>[2x]MKYNTGAGTVPEQLNVHLVPHSHDDVGWLKTVDQYYVGSENYIQEACVENVLDSVVMSLQRDPNRKFVFGEMAFFHRWWLEQTPETKELVRKLVKAGQLEFVNGGWCMHDEATTHYIDMIDHTTLGHRFIQEQFNKIPRAGWQIDPFGHSAVQGYLLGAELGFDSVHFARIDYQDREKRKAEKSLEVVWRGSKTFGSSAQIFANAFPGHYGP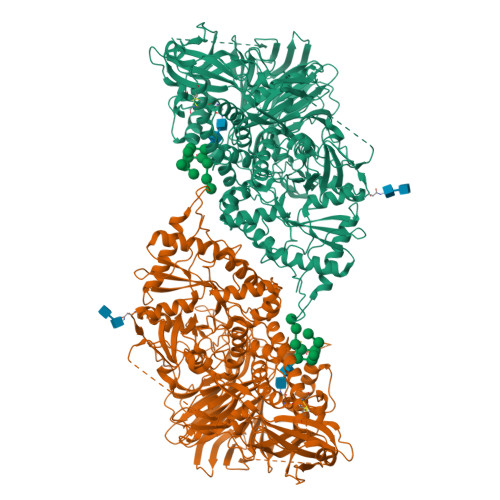PNGFNFEVRNNFVPLQDDPRLFDTNVEERVQNFIDAALTQAKITRTNHIMWTMGDDFQYQYAESWFKQMDKLIHHVNKDGRVNALYSTPSIYTEAKNAANQTWPLKIDDYFPYADGRNAYWTGFYTSRSALKDYVRMLSGYYLATRQLGFFAGKKSTKYHAFDLADALGIAQHHDAVSGTAKQHTTNDYAKRLAIGASKAEAVVSSSLACLTSKQSADQCSAPASAFSQCHLFNISYCPPTESSIPDDKSLVVVVYNPLGWSRNEIVRIPVNDANLVVKDSSGNKLEVQYVEMDDVTANLRSFYVKAYEGEVPKDADVYWSLFKASVPPLGWSTYFISEATGKGTRNALTLSQKGETLNIGPGDLKMSFSSLTGQLKRMYNSKTGVDIPIQQNYLWYESSEGDFSDYQASGAYIFRPNGQPPPHTVSRSSVTRVTRGPLVDEVHQKFNSWISQVTRLYKDKDHAEIEFTIGPIPTDDGVGKEVITRMTSTMATNKEFYTDSNGRDFLKRVRDYREDWPLEVTQPVAGNYYPLNLGIYTKDEKSEFSVLVDRATGGASIKDGEVELMLHRRTIRDDGRGVGEPLDEQVCMNKEYTCEGLTVRGNYYLSIHKPAAGSRWRRTTGQEIYSPMLLAFTQENMENWKSSHSTKGIYMDPNYSLPPSVALITLEELDDGLVLLRLAHLYEPSEDAEYSTLTKVELKKLFATQKIEELREVSLSANQEKSEMKKMKWSVEGDNEQEPQAVRGGPVSNADFVVELGPMEIRTFLLQF>[12x]MKLAVVTGQIVCTVRHHGLAHDKLL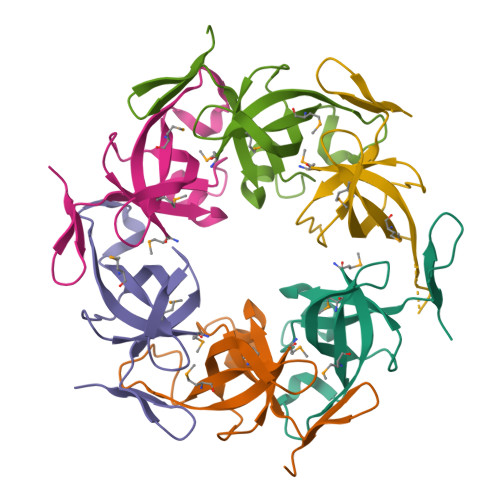MVEMIDPQGNPDGQCAVAIDNIGAGTGEWVLLVSGSSARQAHKSETSPVDLCVIGIVDEVVSGGQVIFHKLEHHHHHH> ADKELKFLVVDDFSTMRRIVRNLLKELGFNNVEEAEDGVDALNKLQAGGYGFVISDWNMPNMDGLELLKTIRANGAMSALPVLMVTAEAKKENIIAAAQAGASGYVVKPFT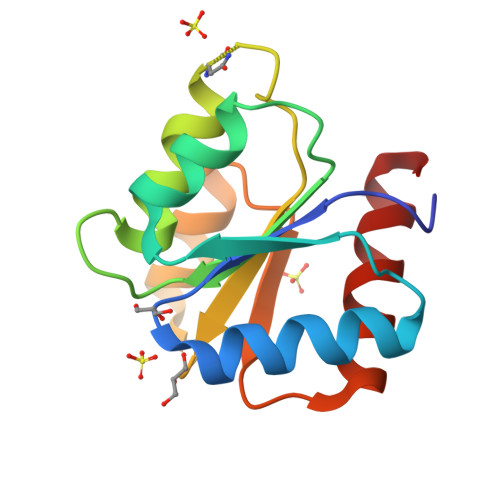AATLEEKLNKIFEKLGM>[6x]MKISIVGAGSVRFALQLVEDIAQTDELSREDTHIYLMDVHERRLNASYILARKYVEELNSPVKVVKTESLDEAIEGADFIINTAYPYDPRYHDSGSQRWDEVTKVGEKHGYYRGIDSQELNMVSTYTYVLSSYPDVKLALEIAEKMK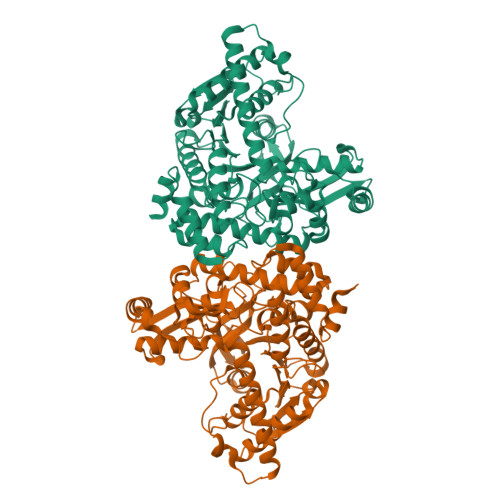KMAPKAYLMQTANPVFEITQAVRRWTGANIIGFCHGVAGVYEVFERLGLDPEEVDWQVAGVNHGIWLNRFRYRGKDAYPLLDEWIEKELSKWEPKNPWDTQMSPAAMDMYRFYGMLPIGDTVRNGTWKYHYNLETKKKWFRRFGGIDNEVERPKFHEHLRRARERLIKLAEEVQENPHLKITEKHPEIFPKGRLSGEQHIPFINAIANNKRVRLFLNVENQGALKDFPDDLVMELPVWVDSSGIHREKVEPDLTHRIKIFYLWPRILRTEWNLEAFISRDRKVLEEILIRDPRTKSYEQVVKVLDEILSLPFNEEIRRYYENLEHHHHHH>MDMTQQEIFDKQRRLQELSEKVRTAHQEISALRKALQ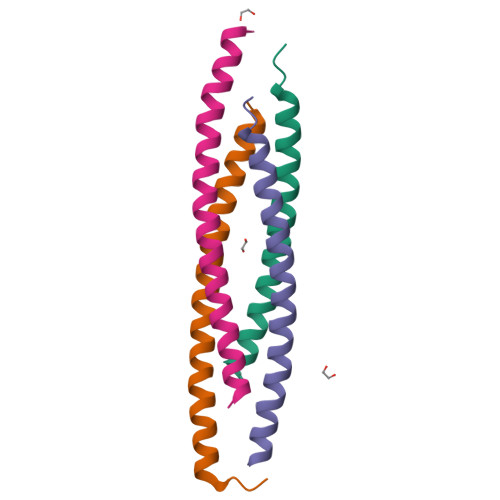EKEAEMLQVLEDIQSI[4x]>MKHHHHHHHGAAGTSLYKKAGENLYFQGSMSLSSWRQFQLFENIPIRDPNFGGDSLLYSDPTLCAATIVDPQTLIIA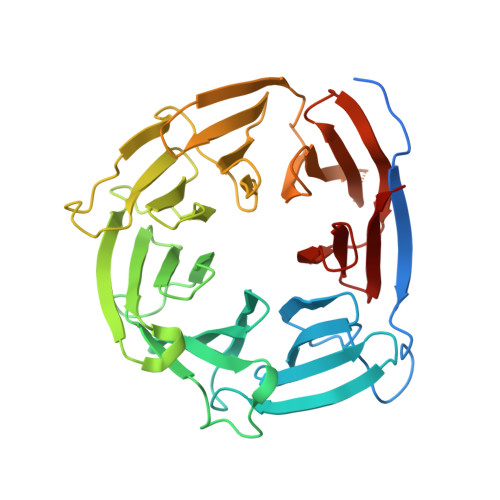VNSNIIKVVKLNQSQVIHEFQSFPHDFQITFLKVINGEFLVALAESIGKPSLIRVYKLEKLPNREQLYHSQVELKNGNNTYPISVVSISNDLSCIVVGFINGKIILIRGDISRDRGSQQRIIYEDPSKEPITALFLNNDATACFAATTSRILLFNTTGRNRGRPSLVLNSKNGLDLNCGSFNPATNEFICCLSNFIEFFSSSGKKHQFAFDLSLRKRIFCVDKDHILIVTEETGVPTTSISVNELSPTIINRIFIIDAKNKIISLNFVVSSAIIDIFSTSQSGKNITYLLTSEGVMHRITPK[3x]>[2x]SSPGKPPRLVGGPMDASVEEEGVRRALDF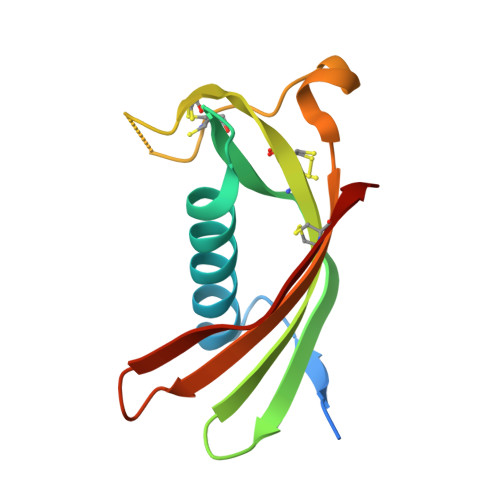AVGEYNKASNDMYHSRACQVVRARKQIVAGVNYFLDVELCRTTCTKTQPNLDNCPFHDQPHLKRKAFCSFQIYAVPWQGTMTLSKSTCQDA>GQDKVECWDRFELSFKQVTKGNPFDIRLSATFVCGKEKKTVEGFYDGENTYRIRFMPAVAGEWRYVTSSSIGAMNGRKGTFTVIPAGKDNHGMVLVDGEHNFKYADGTRYYPMGTTAYAWTHMKETTQEATLKSFGEAGFNKVRMCVFPKNY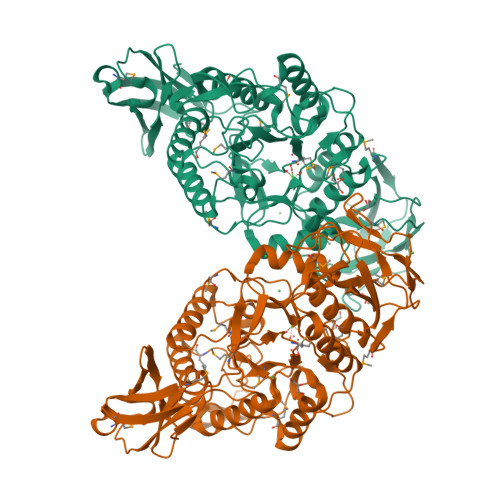SLVKDEPALYPFEIEKTIKDKEGNERKEWDFDRFDPAFFQHLEKRIDQLNRLGIEADLILFHPYDKGRWGFDAMSNEVNVRYIKYITARLASFRNVWWSMANEWDYVKAKTVDDWKLLTKTVVENDPYRHLCSIHGATATYFDYWMPEFTHVSIQDEAPVLSSTASATLRKIYRKPVICDEVGYEGNLPYRWGRLSPQQMTCFILNGLLGGIYVTHGECYQQGNEPIFWAQGGSLKGESWKRVKFLRTIIEAAPHPLEMADISRDLVTSTAGPDYYLVNMGKDVKGFWTFNLPVKNADYNKLQKNKRFKVEIIDVWAMTVTEYPVIFETTEELDYRVFDIHHRGVRIPDAPYIVLRITEVK[2x]> MGSSHHHHHHSQLMVTSTYIPMSQRRSWADVKPIMQDDGPNPVVPIMYSEEYKDAMDYFRAIAAKEEKSERALELTEIIVRMNPAHYTVWQYRFSLLTSLNKSLEDELRLMNEFAVQNLKSYQVWHHRLLLLDRISPQDPVSEIEYIHGSLLPDPKNYHTWAYLHWLYSHFSTLGRISEAQWGSELDWCNEMLRVDGRNNSAWGWRWYLRVSRPGAETSSRSLQDELIYILKSIHLIPHNVSAWNYLRGFLKHFSLP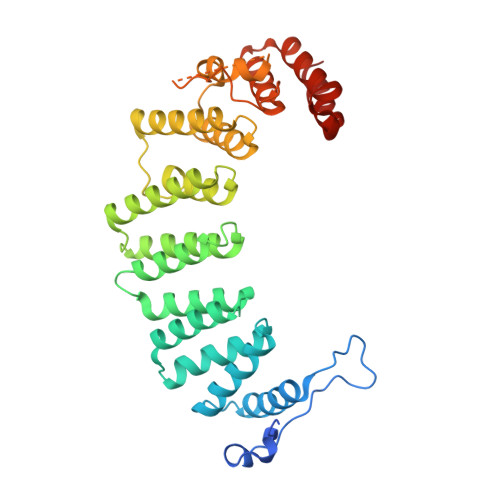LVPILPAILPYTASKLNPDIETVEAFGFPMPSDPLPEDTPLPVPLALEYLADSFIEQNRVDDAAKVFEKLSSEYDQMRAGYWEFRRRECAEE> MAEEKLSARTQLPVSAESQKPVLKKAPEFPILEKQNWLIHLYYIQKDYEACKAVIKEQLQETHGLCEYAIYVQALIFRLEGNIQESLRLFQMCAFLSPQCADNLKQVARSLFLLGKHKAAIEVYNEAAKLNQKDWEICHNLGVCYIYLKQFDKAQDQLHNALHLNRHDLTYIMLGKIFLLKGDLDKAIEIYKKAVEFSPENTELLTTLGLLYLQLGIYQKAFEHLGNTLTYDPTNYKAILAAGSMMQTHGDFDVALTKYKVVACAVIESPPLWNNIGMCFFGKKKYVA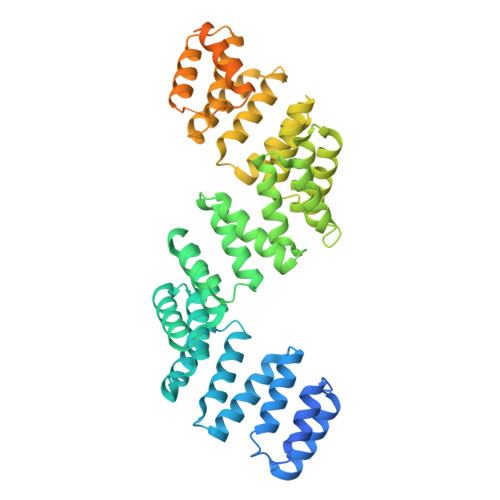AISCLKRANYLAPLDWKILYNLGLVHLTMQQYASAFHFLSAAINFQPKMGELYMLLAVALTNLEDSENAKRAYEEAVRLDKCNPLVNLNYAVLLYNQGEKRDALAQYQEMEKKVNLLKYSSSLEFDPEMVEVAQKLGAALQVGEALVWTKPVKDPKSKHQTASTSKAAGFQQPLGSNQALGQAMSSAATCRKLSSGAGGTSQLTKPPSLPLEPEPTVEAQPTEASAQTREK> MKNNKIYLLGACLLCAVTTFAQNVSLQPPPQQLIVQNKTIDLPAVYQLNGGEEANPHAVKVLKELLSGKQSSKKGMLISIGEKGDKSVRKYSRQIPDHKEGYYLSVNEKEIVLAGNDERGTYYALQTFAQLLKDGKLPEVEIKDYPSVRYRGVVEGFYGTPWSHQARLSQLKFYGKNKMNTYIYGPKDDPYHSAPNWRLPYPDKEAAQLQELVAVANENEVDFVWAIHPGQDIKWNKEDRDLLLAKFEKMYQLGVRSFAVFFDDISGEGTNPQKQAELLNYIDEKFAQVKPDINQLVMCPTEYNKSWSNPNGNYLTTLGDKLNPSIQIMWTGDRVISDITRDGISWINERIKRPAYIWWNFPVSDYVRDHLLLGPVYGNDTTIAKEMSGFVTNPMEHAESSKIAIYSVASYAWNPAKYDTWQTWKDAIRTILPSAAEELECFAMHNSDLGPNGHGYRREESMDIQPAAERFLKAFKEGKNYDKADFETLQYTFER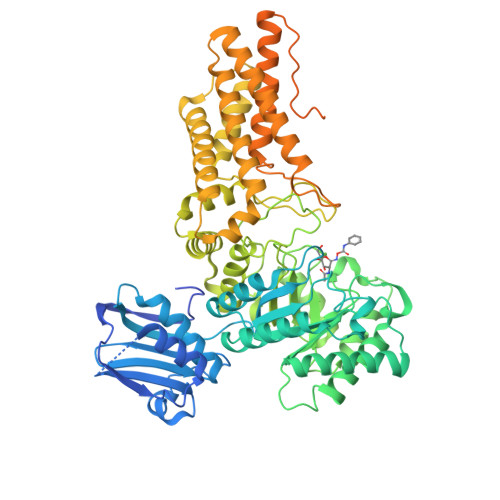MKESADILLMNTENKPLIVEITPWVHQFKLTAEMGEEVLKMVEGRNESYFLRKYNHVKALQQQMFYIDQTSNQNPYQPGVKTATRVIKPLIDRTFATVVKFFNQKFNAHLDATTDYMPHKMISNVEQIKNLPLQVKANRVLISPANEVVKWAAGNSVEIELDAIYPGENIQINFGKDAPCTWGRLEISTDGKEWKTVDLKQKESRLSAGLQKAPVKFVRFTNVSDEEQQVYLRQFVLTIEKK>[4x]MAQLSGQPVVILPEGT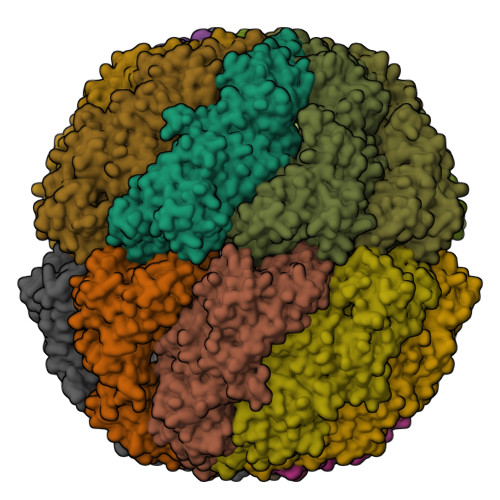QRYVGRDAQRLNILAARIIAETVRTTLGPKGMDKMLVDSLGDIVVTNDGATILDKIDLQHPAAKMMVEVAKTQDKEAGDGTTTAVVIAGELLRKAEELLDQNIHPSIITKGYALAAEKAQEILDEIAIRVDPDDEETLLKIAATSITGKNAESHKELLAKLAVEAVKQVAEKKDGKYVVDLDNIKFEKKAGEGVEESELVRGVVIDKEVVHPRMPKRVENAKIALINEALEVKKTETDAKINITSPDQLMSFLEQEEKMLKDMVDHIAQTGANVVFVQKGIDDLAQHYLAKYGIMAVRRVKKSDMEKLAKATGAKIVTNVKDLTPEDLGYAEVVEERKLAGENMIFVEGCKNPKAVTILIRGGTEHVIDEVERALEDAVKVVKDVMEDGAVLPAGGAPEIELAIRLDEYAKQVGGKEALAIENFADALKIIPKTLAENAGLDTVEMLVKVISEHKNRGLGIGIDVFEGKPADMLEKGIIEPLRVKKQAIKSASEAAIMILRIDDVIAAKATKPEGGQGGGMPGGMGGMDMGM>MAHHHHHHMPRITQEISYNCDYGDNTFNLAIDIGGTLAKVVFSPIHSNRLMFYTIETEKIDKFMELLHSIIKEHNNGCYRMTHIIATGGGAFKFYDLLYENFPQIKGISRFEEMEGLIHGLDFFIHEIPDEVFTYNDQDGERIIPTSSGTMDSKAIYPYLLVNIGSGVSILKVTEPNNFSRVGGSSLGGGTLWGLLSLITGAQTYDQMLDWAQEGDNSSVDMLVGDIYGTDYNKIGLKSSAIASSFGKVFQNRMTSNKSLENNENKLYSSHESIEKNNGQMFKNPDICKSLLFAISNNIGQIAYLQAKINNIQNIYFGGSYTRGHLTTMNTLSYAINFWSQGSKQAFFLKHEGYLGA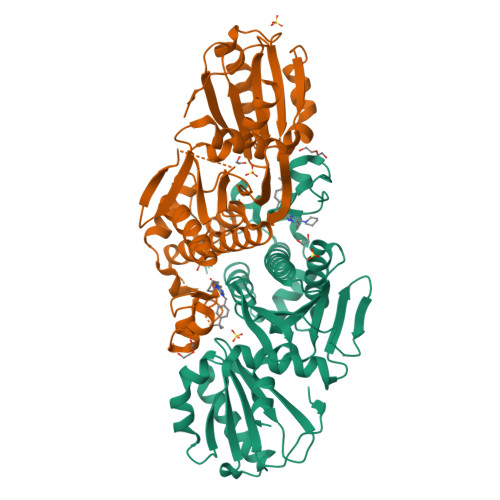MGAFLSASRHSSTKKTST[2x]Innate immune antagonism of RVFV is primarily mediated by its main virulence factor, the 30 kDa non-structural protein (NSs), which is transcribed and translated from a subgenomic mRNA derived from the antigenomic S segment early during infection. NSs impedes interferon production through three known mechanisms. A characteristic feature of RVFV pathogenesis is formation of 0.5 μm thick proteinaceous filaments formed by bundles of thin fibrils in the nuclei of infected cells. Here we describe the first high-resolution structure of a bunyaviral NSs protein.

A truncated stable, soluble core domain spanning residues 83–248 of RVFV NSs (NSs-ΔNΔC) was identified using NMR spectroscopy. The crystals were found to be extremely fragile, and diffracted synchrotron X-rays to 2.2 Å resolution. The structure was successfully phased from the anomalous sulfur signal in a single native crystal and refined to high quality. The NSs-ΔNΔC monomer, molecular mass 19,029 Da, measures approximately 30 × 30 × 50 Å. It is composed of eight α-helices with helices α1-α6 and α8 arranged around a long central helix α7. Two NSs-ΔNΔC monomers constitute the asymmetric unit, with an interface formed by their α8 helices. We therefore conclude the NSs-ΔNΔC structure represents a novel fold. In the crystal lattice NSs-ΔNΔC molecules were found to pack into a highly organized network of two fibril-like assemblies, referred to here as F1 and F2, creating large solvent channels. The T1 interface perpendicular to the F1 fibril axis is defined by an extensive network of hydrogen bonds and salt bridges between the basic face of α1 (Lys84, Gln87, Arg88) and the acidic face of α8 (Glu220, Glu221, Ser228), leading to a large buried interface area of 4 × 852 Å2. Therefore, we conclude that the F1 crystal fibril is not only more stable than F2, but that it also represents the architecture of NSs in intranuclear filaments.

>[2x]GAMVAKPFQRLIDLIGHMTLSDFTRFPNLKEAISWPLGEPSLAFFDLSSTRVHRNDDIRRDQIATLAMRSCKITNDLEDSFVGLHRMIATEAILRGIDLCLLPGFDLMYEVAHVQCVRLLQAAKEDISNAVVPNSALIVLMEESLMLRSSLPSMMGRNNWIPVIPPIPDV>MKSPEELKGIFEKYAAKEGDPNNLSKEE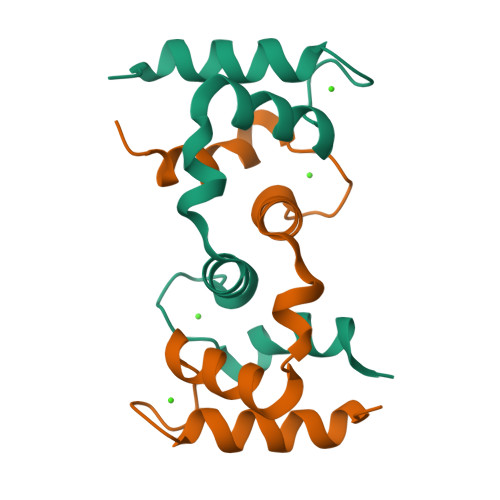LKLLLQTEFPSLLKGMSTLDELFEELDKNGDGEVSFEEFQVLVKKISQ[2x]>[2x]A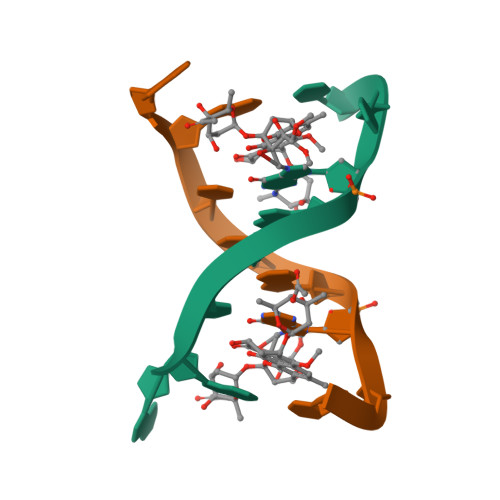ACCGGTT> ANGQSTRYWDCCKPSCGWRGKGPVNQPVYSCDANFQRIHDFDAVSGCEGGPAFSCADHSPWAINDNLSYGFAATALSGQTEESWCCACYALTFTSGPVAGKTMVVQSTSTGGDLGSNHFDLNIPGGGVGLFDGCTPQ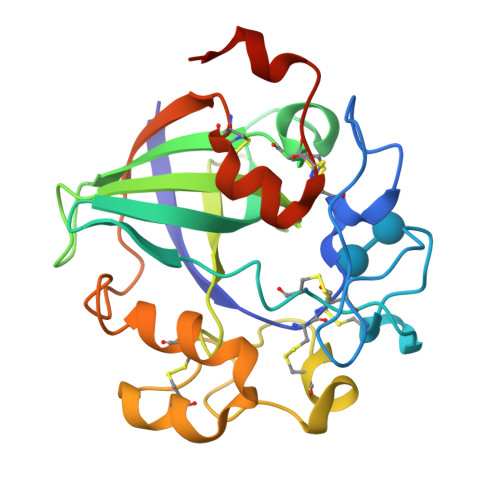FGGLPGARYGGISSRQECDSFPEPLKPGCQWRFDWFQNADNPSFTFERVQCPEELVARTGCRRHDDGGFAVFKAPSA>ETKFVQALFDFNPQESGELAFKRGDVITLINKDDPNWWEGQLNNRRGIFPSNYVCPYNSN[2x];>P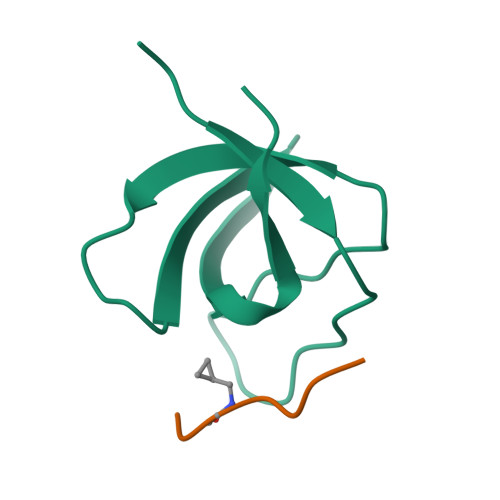PPVGPRRR[2x]>[2x]GPLSLSVDAFKILEDPKWEFPRKNLVLGKTLGEGEFGKVVKATAFHLKGRAGY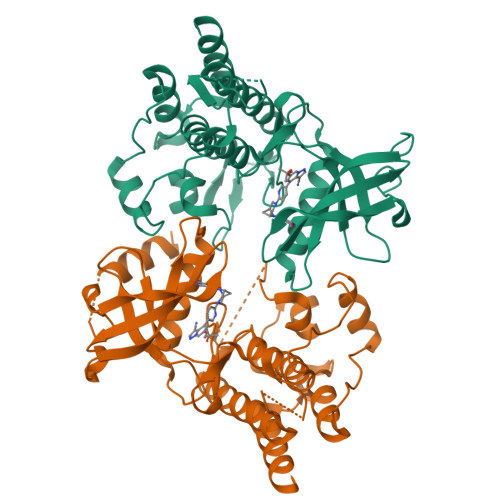TTVAVKMLKENASPSELRDLLSEFNVLKQVNHPHVIKLYGACSQDGPLLLIVEYAKYGSLRGFLRESRKVGPGYLGSGGSRNSSSLDHPDERALTMGDLISFAWQISQGMQYLAEMKLVHRDLAARNILVAEGRKMKISDFGLSRDVYEEDSYVKRSQGRIPVKWMAIESLFDHIYTTQSDVWSFGVLLWEIVTLGGNPYPGIPPERLFNLLKTGHRMERPDNCSEEMYRLMLQCWKQEPDKRPVFADISKDLEKMMVKRR>AEIGGDHGYNATNIAAGQTSGAVTQIGPAVMGMVRRAIPNLIAFDICGVQPMNSPTGQVFALRAVYGKDPVAAGAKEAFHPMYGPDAMFSGQGAAKKFPALAASTQTTVGDIYTHFFQETGTVYLQASVQVTIDAGATDAAKLDAEIKKQMEAGALVEIAEGMATSIAELQEGFNGSTDNPWNEMGFRIDKQVIEAKSRQLKAAYSIELAQDLRAVHGMDADAELSGILATEIMLEINREVVDWINYSAQVGKSGMTLTPGSKAGVFDFQDPIDIRGARWAGESFKALLFQIDKEAVEIARQTGRGEGNFIIASRNVVNVLASVDTGISYAAQGLATGFSTDTTKSVFAGVLGGKYRVYIDQYAKQDYFTVGYKGPNEMDAGIYYAPYVALTPLRGSDPKNFQPVMGFKTRYGIGINPFAESAAQAPASRIQSGMPSILNSLGKNAYFRRVYVKGI[6x];>[2x]MTFTVDITPKTPTGVIDETKQFTATPSGQTGGGTITYAWSVDNVPQDGAEATFSYVLKGPAGQKTIKVVATNTLSEGGPETAEATTTITVKNKTQTTTLAVTPASPAAGVIGTPVQFTAALASQPDGASATYQWYVDDSQVGGETNSTFSYTPTTSGVKRIKCVAQVTATDYDALSVTSNEVSLTVNKKTMNPQVTLTPPSINVQQDASATFTA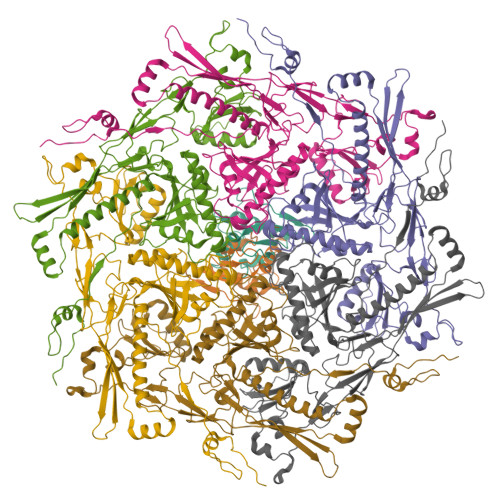NVTGAPEEAQITYSWKKDSSPVEGSTNVYTVDTSSVGSQTIEVTATVTAADYNPVTVTKTGNVTVTAKVAPEPEGELPYVHPLPHRSSAYIWCGWWVMDEIQKMTEEGKDWKTDDPDSKYYLHRYTLQKMMKDYPEVDVQESRNGYIIHKTALETGIIYTYP>SNAMKQAIGFIDSGVGGLTVVREVLKQLPHEQVYYLGDTARCPYGPRDKEEVAKFTWEMTNFLVDRGIKMLVIACNTATAAALYDIREKLDIPVIGVIQPGSRAALKATRNNKIGVLGTLGTVESMAYPTALKGLNRRVEVDSLACPKFVSVVESGEYKSAIAKKVVAESLLPLKSTKIDTVILGCTHYPLLKPI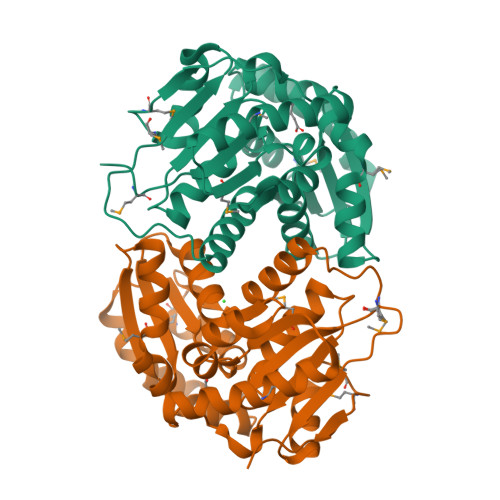IENFMGDGVAVINSGEETASEVSALLDYHNLLDATDEEIEHRFFTTGSTQIFKDIAKDWLNMPDMTVEHIKLGK[2x]>MIVFVRFNSSHGFPVEVDSDTSIFQLKEVVAKRQGVPADQLRVIFAGKELRNDWTVQNCDLDQQNIVHIVQRPWRKGQEMNATNSFYVYCKGPCQRVQPGKLRVQCSTCRQATLTLTQGPSCWDDVLIPNRMSGECQSPHCPGTSAEFFFKCGAHPTSDKETSVALHLIATNSRNITCITCTDVRSPVLVFQCNSRHVICLDCFHLYCVTRLNDRQFVHDPQLGYSLPCVAGCPNSLIKELHHFRILGEEQYNRYQQYGAEECVLQMGGVLCPRPGCGAGLLPEPDQRKVTCEGGNGLGCGFAFCRECKEAYHEGECSAVFEASGTTTQAYRVDERAAEQARWEAASKETIKKTTKPCPRCHVPVEKNGGCMHMKCPQPQCRLEWCWNCGCEWNRVCMGDHWFDV[2x]

Mutations in genes encoding PTEN-induced kinase 1 (PINK1) (human PARK6) and the ubiquitin E3 ligase Parkin (human PARK2) are causal for early onset Parkinson's disease (PD) with clinically indistinguishable phenotypes. PINK1 directly phosphorylates Parkin at a highly conserved serine 65 (Ser65) residue within its N-terminal ubiquitin-like domain (Ubl), as well as the equivalent Ser65 residue of ubiquitin (Ub). Phosphorylation of both Parkin and ubiquitin is required for maximal activation of Parkin E3 ligase activity. Upon activation, Parkin ubiquitylates multiple substrates at the OMM leading to both de novo assembly and elongation of existing ubiquitin chains that are, in turn, phosphorylated by PINK1.

Here we report the first clinical and genetic evidence of PD associated with homozygous mutations at p.S65N, the critical node of the PINK1–Parkin pathway. To understand precisely how the pathogenic S65N mutation affects Parkin activity, we crystallized and solved the structure of the novel human Parkin PD mutant (UBLR0RBR, Δ84–143) at 2.9 Å. Comparative analyses of wild-type and ParkinS65N x-ray crystal structures did not reveal any conformational differences between the wild-type and mutant protein, indicating that the S65N mutation does not significantly perturb Parkin structure. However, as the S65N mutation prevents incorporation of a phosphate group at this position, the absence of a negative charge at the UBL-IBR interface inhibits the ability of ParkinS65N to adopt the open conformation required for full E3 activity. This contrasts to wild-type Parkin, where phosphorylation at Ser65 induces key conformational changes and new interactions. Immunoblotting of protein extracts demonstrated that the S65N mutation was functionally equivalent to the S65A mutation, leading to both a loss of both Parkin activation (as judged by reduced CISD1 and Miro1/2 substrate ubiquitylation) and reduced phospho-ubiquitin accumulation. Immunoblotting with anti-phospho-Ser65 Parkin antibodies demonstrated that Parkin phosphorylation was abolished in cells expressing S65N. This was associated with substantial reduction of Parkin E3 ligase activity as judged directly by ubiquitylation of CISD1 in PARKINS65N/S65N fibroblasts. The probe revealed robust labelling of activated wild-type human Parkin in control fibroblasts, whereas this was completely disrupted in PARKINS65N/S65N mutant fibroblasts. Characterization of patient-derived primary cells demonstrates that the Parkin S65N mutation is inactive, suggesting that the loss of PINK1-dependent Parkin Ser65 phosphorylation and subsequent inactivation in humans is sufficient to cause PD.> GSAY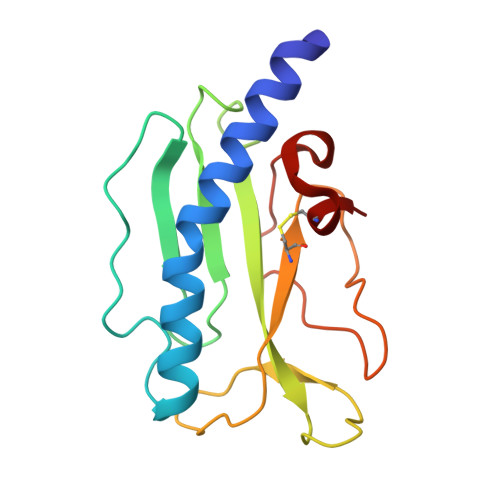QDYLARSRVGEGLALAASARLAVAENAASGNGFSGGYVSPPATRNVDSIRVDDDSGQIVVAFTTRVAAAGANTLVLVPSAPDQADTPTARVALSKGAVQAGAITWECFADGKASSSLPAPGAGPLPTDAPTLAGKLAPPECRA>[12x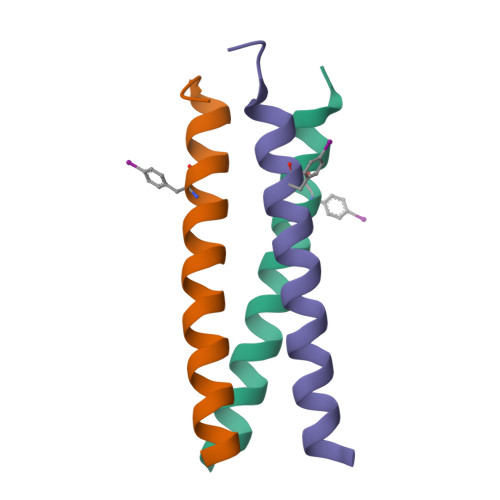]XGEIAAIKQEIAAIKKEIAAIKFEIAAIKQGYG>[4x]MVELTPAAIQELERLQTHGVRRGQAAILRIQVQPSECGDWRYDLA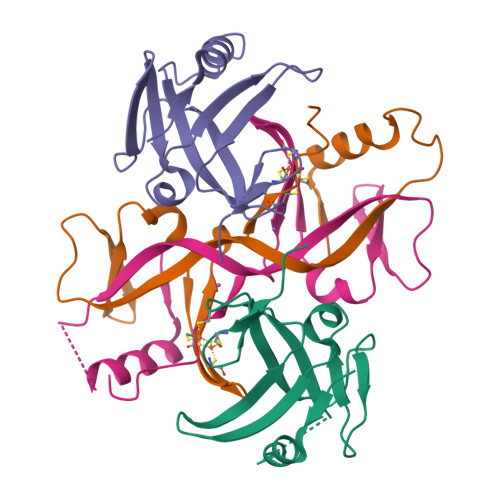LVAEPKPTDLLTQSQGWTIAIAAEAAELLRGLRVDYIEDLMGGAFRFHNPNASQTCGCGMAFRVSRS>[2x]MSTVRRLEGKVALITGGAGNIGEVITRRFLAEGATVVITGRNAEKLAVYRRRLIDEERVAPERVVALRMDGSDIAQVRAGVAQIVHGGTDVPIPLHRIDILVNNAGSAGPRRRLVDIPLEPSEVQPPDSETLAQAVGNLVGITWNLTRAAAPHMPSGSSVINISTIFSRTDYYGRIAYVAPKAALNALSDGLARELGVRGIRVNTIYPGPIESERIYTMFQAMDALKGQPEGDTASGFLRMMRLSRIDQNGEVVKRFPSPVDVANTAVLLASDESAAFTGHAFEVTHGMEVPTESRTTFVSRPGLRSVDATGKVILICAGDQVDDAVALADTLRSCRATVVIGFRDPRALEKASVLLREPRHALAADMYGRPTMTAEARLVRLDPLDPRAAAQTLEQIHAELGAIHHAVVLPGQSRHAPSASLIEVDDQVVERFLHQELVGTIALARELARFWEEYPSGSSMHRVLFVSNPDDQQGNQYSHILRAAVEQLVRVWRHESEYDSVNPAHQQEGQSSAAVWANQLIRYVNNEMANLDFTCAWVAKLLGSDRRIAEINLYLPEEIVGTIGVHNPGFGWAESLFGLHMGKVALITGGSAGIGGQIGRLLALSGAHVMLAARNADQLEQMRASIVREVRDASYPDAESRVAIFPGSDVSDIDGLERLVNHTVRVFGKVDYLINNAGIAGAEEMVIDMPVDAWRHTLRANLISNYALLRRLAPQMKAAGGAYVLNVSSYFGGEKYVAIPYPNRSDYAVSKAGQRAMVESLARFLGPEIQINAIAPGPVEGERLKGAGSRPGLFMRRARLILENKRLNEVFAALLAARHEGATIADLLPDLFANDIQSIANSAAMPAPLRRLATMLRETSDAGGSAQSYLMNATIARKLLNRLENGGYITLHDRRALTVEPPEPFFTEAQIEREAIKVRDGILGMLHLQRMPTEFDVALATVFYLADRNVTGETFHPSGGLRFERTVTEGELFGKPGQQRLERLKGSVVYLIGEHLRQHLVLLARTFLDEIHVARVVLLTETTQAATDLAAELSDYEAAGRFVVIPTCGDIEGGIDRAMAEYGRPGPVISTPFRPLPDRALSARNGDWSSVLTTAEFEELVEQQITHHFRVARKAGLIEGANVTLVTPPTSARSTSEEFALANFVKTTLHALTATAGAESERTVPHVPVNQVDLTRRARSEEPRTPSEEEEELQRFVNAVLLTSAPLPTPLESRYRARIYRGNAITV

Malonyl-CoA reductase (MCR) is a NADPH-dependent bi-functional enzyme that performs alcohol dehydrogenase and aldehyde dehydrogenase (CoA-acylating) activities in the N- and C-terminal fragments, respectively. It catalyzes the two-step reduction of malonyl-CoA to 3-hydroxypropionate (3-HP), a key reaction in the autotrophic CO2 fixation cycles of Chloroflexaceae green non-sulfur bacteria and the archaea Crenarchaeota. In contrast, green non-sulfur bacteria, including members of the genera Chloroflexus and Roseiflexus, employ a single bi-functional MCR to catalyze both reduction reactions of malonyl-CoA. Full-length RfxMCR was a homodimer of two cross-interlocked subunits, each containing four tandemly arranged short-chain dehydrogenase/reductase (SDR) domains.

For the first time, we here determined the cryo-electron microscopy (EM) structure of the full-length MCR from Roseiflexus castenholzii (RfxMCR), which shares 58% sequence identity with CfxMCR, at 3.35 Å resolution. To investigate the dimer structure, RfxMCR was imaged on a 300 kV Titan Krios cryo-EM with a K3 Summit direct electron detector (Gatan) in counting mode. From 4,647 micrographs, 4,043,667 particles were selected and used to construct an electron potential map with an average resolution of 3.35 Å (Fig. S1D through G). The overall structure of RfxMCR was a homodimer of two cross-interlocked subunits with the N- and C-terminal ends assembled in the same direction; the dimensions were 160 × 110 × 95 Å. The ED (Gly783–Arg932), which comprised eight α-helices, was inserted into the SDR3 domains (Gly573–Glu782 and Met933–Gly962) and was exposed at the two sides of the homodimer. From the full-length RfxMCR structure, we first resolved the conformation of RfxMCR-N and RfxMCR-C connecting region, which was folded into an α-helix (G573WAESL578). In the center of the homodimer, two of these α-helices were anti-parallel arranged in the reverse direction. Instead, it plays an important role in connecting the RfxMCR-N and RfxMCR-C fragments and also serves as a point of intersection for the two subunits to form a dimer. Actually, the dimer interface was formed by symmetrically distributed hydrogen bonding interactions between amino acid residues from the RfxMCR-N (SDR1–SDR2) and RfxMCR-C (SDR3–ED–SDR4) of the two subunits. We did not resolve any densities of substrate or cofactor from the cryo-EM maps of full-length RfxMCR incubated with NADP+ or malonyl-CoA.> GPLGSMVDYIVEYDYDAVHDDELTIRVGEIIRNVKKLQEEGWLEGEL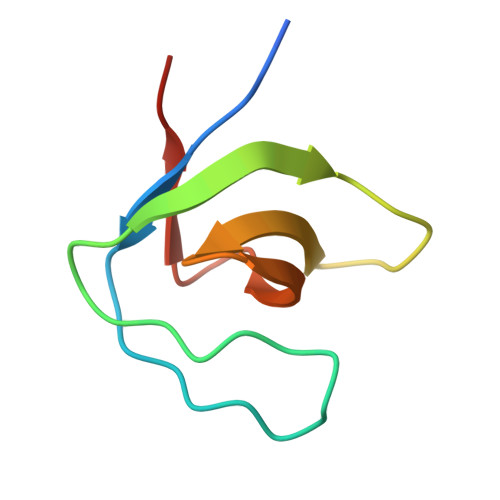NGRRGMFPDNFVKEIKRE> AGAGADRTAATPAAANPAATEPVKWECPAGYEVKEGLNVDFPHKGMKRAFIVYPAKNVSGPAPVWVPMTGSVESTNDNLTVARSGANSILADHGYTVIA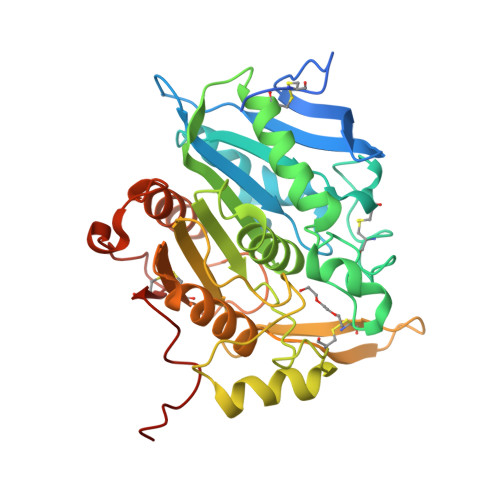PVRACANQDPNIRGERCNGPGSNGWNWNPWFEGRAADPSGEHWKNDEGPDSSFFVAMVQCVGTKYKLDARRLFLGGISSGGTMTNRALLFRSNFWAGGLPISGEWYVTSDDGTPLSFDDARAAVAAAPTKIHQGRVGPYPLPAKVGPLIVMTVWGGEKDLWNCTRPDGSRFLCADYRPSTQAGSNFFSAQPDVVHVACSSTHGHMWPQLNTQEFNRWALDTLASHPKGSDPRSFKLTQPPEGYTCHVGPFTGLYASAWSHPQFEK>[14x]MNLIPTAIETTNRGERAYDIYSRLLKDRIIMLGSQIDDNVANSIVSQLLFLQAQDSEKDIYL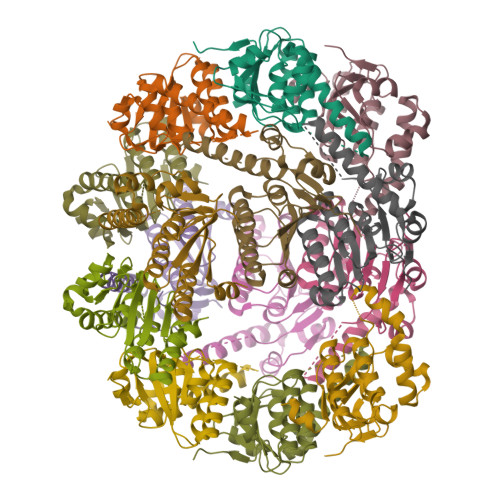YINSPGGSVTAGFAIYDTIQHIKPDVQTICIGMAASMGSFLLAAGAKGKRFALPNAEVMIHQPLGGAQGQATEIEIAANHILKTREKLNRILSERTGQSIEKIQKDTDRDNFLTAEEAKEYGLIDEVMVPETK4-NITROPHENYL 4-O-ALPHA-D-GLUCOPYRANOSYL-ALPHA-D-GALACTOPYRANOSIDE | C18 H25 N O13 | 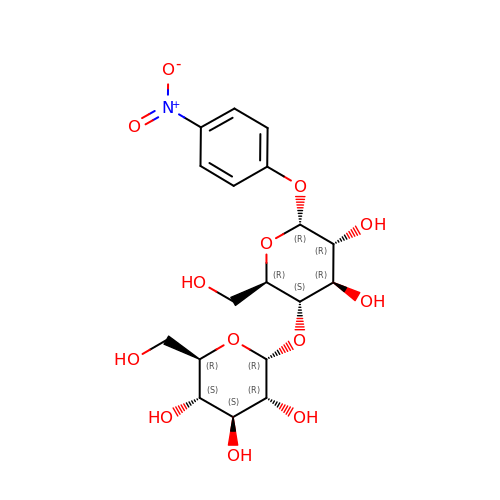IAYJZWFYUSNIPN-LTHBGAKLSA-N> MFNFFSSANINQNIPKYSVNDFVFRLKKIEKIVVKEGLDG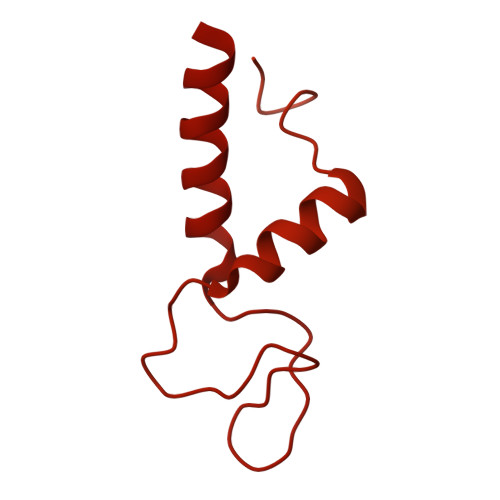FLLINGVDSRENTEYVKLTNWLFLGNSGLEIEENEYLNQIYSDMIVLIKKGTTHIFIDPEALNSLQTLIYSIPNVDVFCPTEKQYEDKDEMELLKMAFFLRVMKPTKKVGILLGQKDKGKINSIEKWPLIQSYGLEELGVGFFSMNHEVVDLTLRLNAVYKNYDKFFVSKLIYVVAKRLTGHFNSAAGQLGDMKMHKRNLATESQLTEIFRDTYEIEEISKWVQIRGVNAALPKPRVLFGKNTSADCSKEPSVAPLKDLKYSETFHSFHATFETFDLRTCLRAARTYFLAKGVKEERNLITLNDDEGVPQGYELNIDENQQYKDQDFLANLYLSIIIGFNEVMQLITKDYKNMTEEFIQDYIFQKVSKVYAGFQIPESEITLDKIQIILKAYNSFGEEVKIDFKDTISFKLTPYFFMVRIEQKNIKSQILNNTVLGSLVFAESFILQEGCYLLLTKEIPYFDLWNCQNDYSEKIEKMKKRILWEPLGKQISDELPKNRIFVQTGRKSNYGFDIPIMQASYYMHELGLRIETQRLGWFILFFKEMKEIQITQKMNHTWLIFKVDSNITFNSISKDTIALEFTGDALEQSFFKIKNYFEENQIKYEYQVDIPAIFQESQIAKKQILNQQSQGQKLITMNSIQNEQFFISYIESKQLMILNQMKDLKLSAYKNLYEQMQISQAITPVENHIGVILVNGSYCSGKRKFAENLIRFGSDNNLRLHLYKFDLNEMSELTEKSYLSGLLKFASEKKIQNTDVIVASVPHFINTKILIDYFSKSEKISNAFYIRTIATKININNIYSNFNKNPVNNVFTYGVEGYSQFLLLDTYNNYDADVNALNKTLSGVLPGAKIYKIMNNILNPALAKDILTSITFISEQNNLNRLKYSVQYDLLTSNGPSSVVFIPFKLPILREKIRDLIYKKILQNGNQTLVDTIEAEQKIAEFKELNKNSKDPLMIEIIKLKEKIEIQNAQTSDQAIKIDYVKGILRYDSKLKEGLEEITITPNYFIERTVKGVDAKEFTEELNGVSFKNVKYTGITNSIINDMGFVFAGKNLNKEKLLELLYKLVKPLNKQKLRQRKDLTEEEIVDIQFRNRGEGLENGEFYDGQFWRNIQGLILPHHPKKDEFIEEYLKQEEVRINQINEQLQQEWETWKQVYDKIHLDK> GAGCAGCCTGTCTGGACATCA;> CCAUACA;> GGCTGCT;> CTGA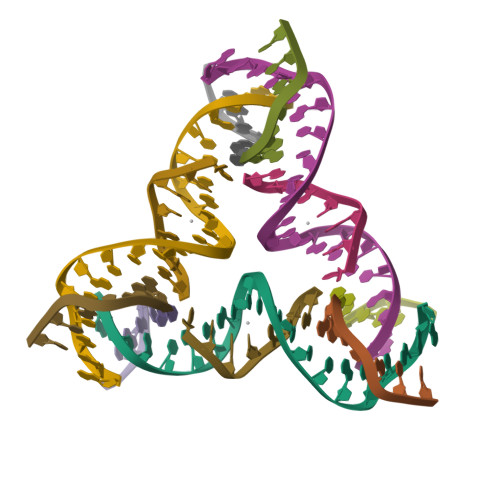TGT> GHMVKSGLQIKKNAIIDDYKVTSQVLGLGINGKVLQIFNKRTQEKFALKMLQDCPKARREVELHWRASQCPHIVRIVDVYENLYAGRKCLLIVMECLDGGELFSRIQDRGDQAFTEREASEIMKSIGEAIQYLHSINIAHRDVKPENLLYTSKRPNAILKLTDFGFAKETTGHNSLTTPCYTPYYVAPEVLGPEKYDKSCDMWSLGVIMYILLCGYPPFYSNHGLAISPGMKTRIRMGQYEFPNPEWSEVSEEVKMLIRNLLKTEPTQRMTITEFMNHPWIMQSTKVPQTPLHTSRVLKEDKERWEDVKEEMTSALATMR

We aimed to develop covalent inhibitors targeting tyrosine residues in the protein kinases JAK3 and MK2 using structure-based design principles to generate small sets of ligands containing tyrosine-reactive sulfonyl fluoride and the less-explored fluorosulfate warheads. By utilizing a structure-based approach with well-characterized kinases, we focus on Janus kinase 3 (JAK3) and mitogen-activated protein kinase-activated protein kinase 2 (MK2, also known as MAPKAPK2) as model targets. In conclusion, we successfully synthesized a small but diverse set of novel fluorosulfate and sulfonyl fluoride warhead-bearing compounds, initially designed to covalently target tyrosine residues in both JAK3 and MK2 using structure-based design principles.

MK2, a serine/threonine kinase activated by the p38 MAP kinase, plays a critical role in the cellular stress response, inflammation, and regulation of pro-inflammatory cytokines. While compound 43 (bearing a fluorosulfate next to the piperazine) showed no binding in our experiments, 64 (the sulfonyl fluoride analogue) showed 15% covalent modification of the protein and compound 42 (bearing a fluorosulfate next to the chloride) displayed an impressive 95% covalent binding to MK2 within the time frame of the experiment. To determine the exact location of the covalent modification, we solved an X-ray crystal structure with the most efficient covalent binder, compound 42, in complex with MK2. To our surprise, 42 does not bind into the allosteric pocket at all but rather occupies the ATP binding site where it reacts with the “catalytic” lysine, Lys93. The reason for the poor activity seen in enzymatic assays despite an orthosteric binding mode may reside in the relatively slow inactivation kinetics of fluorosulfates which may not compensate for a relatively weak non-covalent affinity on the assay time scale and under ATP-competitive conditions. Consistent with this, the measured kinact/KI value of 1.12 M−1 s−1 (see also the ESI†) confirms the low overall efficiency of covalent binding process, supporting the hypothesis that the weak non-covalent affinity and slow inactivation kinetics limit the compound's activity. Beyond the covalent interaction, the hinge binding mode of this compound is also intriguing: since the inhibitor was not designed to be orthosteric, it does not contain an obvious hinge binding motif. Instead, the carbonyl oxygen of the amide bond interacts with the backbone amine of Leu141, similar to the hinge interaction observed for skepinone-type inhibitors of the upstream kinase p38α,66 yet without the peptide flip induced by the latter. In our second tyrosine targeting study, unexpectedly, one of the putative allosteric MK2 inhibitors formed a covalent bond with the “catalytic” lysine, showcasing an unanticipated binding mode not just in its covalent interaction but also in the atypical interaction of the carbonyl group with the hinge region.>GIDPFTMNAKPGFTDYIVKDIALADFGRKEISLAETEMPGLMATREEYGPKQPLKGARIAGSLHMTIQTAVLIETLAALGADIRWVSCNIYSTQDHAAAAIAAAGIPVFAVKGETLTEYWDYTAKLFDWHGGGTPNMILDDGGDATMLVHAGYRAEQGDTAFLDKPGSEEEEIFYALVKRLLKEKPKGWFAEIAKNIKGVSEETTTGVHRLYEMANKGTLLFPAINVNDSVTKSKFDNLYGCRESLVDGIRRGTDVMLSGKVAMVAGFGDVGKGSAASLRQAGCRVMVSEVDPICALQAAMEGYEVVTMEDAAPRADIFVTATGNKDIITIEHMRAMKDRAIVCNIGHFDNEIQIASLRNLKWTNIKPQVDEIEF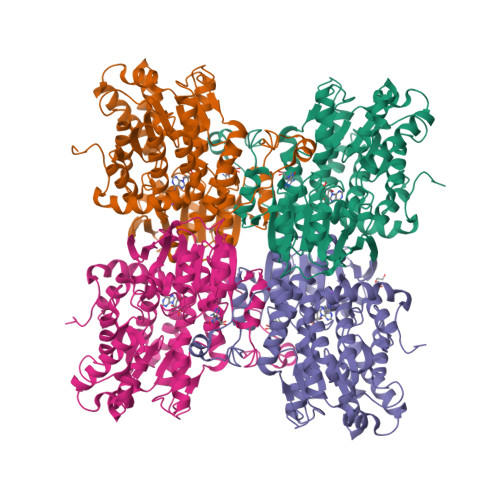PDKHRIIMLSEGRLVNLGNAMGHPSFVMSASFTNQTLAQIELFANNKDSKYAKKVYVLPKTLDEKVARLHLAKIGVKLTELRKDQADYIGVKQEGPYKSDHYRY[4x]> MFKYLTPIFLCTAAISFQAQADDTMLMLLKKDNATYLSWSTDAGNVVRQDVYRSTSSAQAGSEKIAELNSSDRTFTDLTANPQSDYWYWVDTVSGNNSVLKSNAASTAPAPLRAAPLKAASPECKAGAVIKDKTVDCGGITLGLSCSGDSDKQPPVITLENATIKNL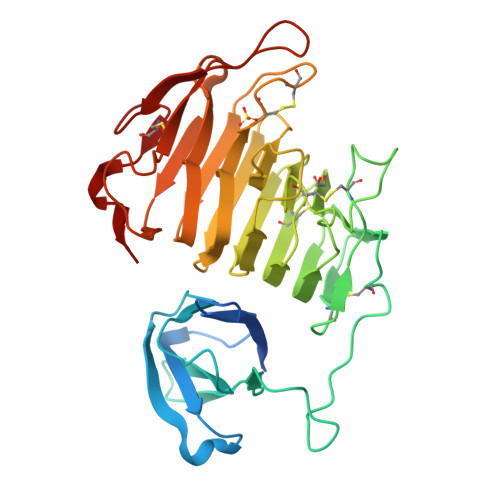RISEKGGSDGIHCKSGNCRIENVIWEDICEDAATNLGKTMTIVGGVAHNTTNGPGGKPDKVLQQNAKNSHTIVQGNFTLTGQHGKLWRSCGDCTNNGGPRNLTIISATVNGTIDSIAGVNRNFGDVAEIRDLRIKGYKEGKPPVCEEFNGVEKGKGKSDKYGEFWDTKNCKVSRSNVKPL>[4x]GMGKRDDLIAQYADDLRNKCGMEPDMALLEKVTKGCGPA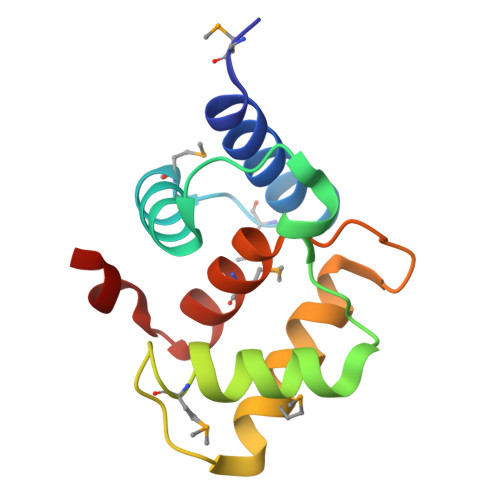IYNRDASTVAGSDTAELETIKKNFLMKKLGLADSESLMGGIQSVIETYGRSERNKYRAVVYYMLTKHFGKESVYG>SNAMRIGHGFDVHAFGGEGPIIIGGVRIPYEKGLLAHSDGDVALHALTDALLGAAALGDIGKLFPDTDPAFKGADSRELLREAWRRIQAKGYTLGNVDVTIIAQAPKMLPHIPQMRVFIAEDLGCHMDEVNVKA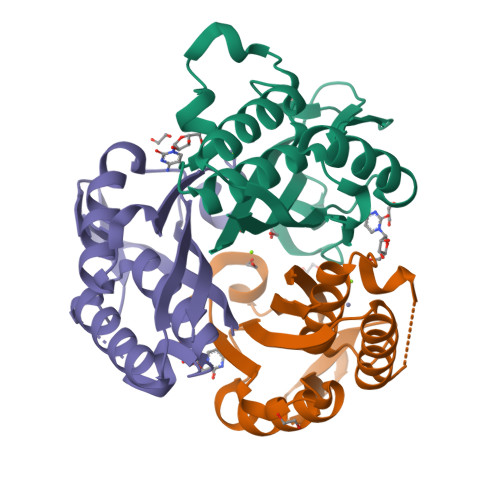TTTEKLGFTGRGEGIACEAVALLMKAAK[6x]>[4x]GPLGSMSQSNRELVVDFLSYKLSQKGYSWSQMAAVKQALREAGDEFELRYRRAFSDLTSQLHITPGTAYQSFEQVVNELFRDGVNWGRIVAFFSFG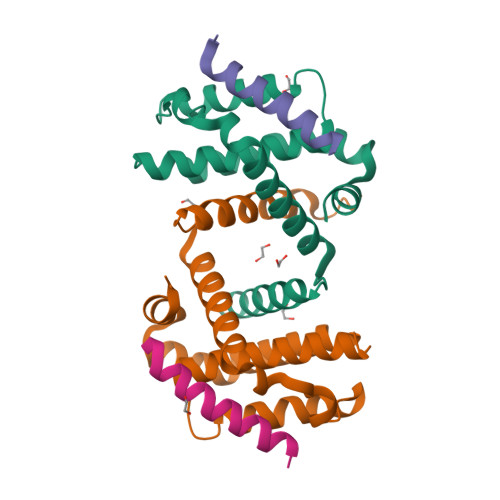GALCVESVDKEMQVLVSRIAAWMATYLNDHLEPWIQENGGWDTFVELYGNNAAAESRKGQER;>[4x]DMRPEIRIAQELRRXGDEFNATYARR Entry of a hantavirus into a host cell is negotiated by two membrane-anchored glycoproteins, Gn and Gc, which form a lattice decorating the lipid bilayer envelope of the mature virion. The Gc adopts a three-domain (domains I−III) class II fusion protein architecture and is postulated to associate closely with the Gn, linking adjacent Gn tetramers. Endosomal escape is mediated by the Gc in a process that involves engagement of the target membrane by the Gc-encoded fusion loop, followed by upward ‘zippering action’ conformational rearrangements of the transmembrane-anchored Gc domain III, which bring together host and viral membranes. Here we structurally characterize the epitope of mAb P-4G2, a potently neutralizing antibody derived following experimental infection of bank voles with Puumala virus (PUUV), a hantavirus responsible for one of the most frequently occurring hantaviral diseases, a mild form of HFRS known as nephropathia epidemica (NE).

To ascertain the position of the P-4G2 epitope in the context of the hantaviral envelope, we generated PUUV virus-like particles (VLPs) by transient expression of the PUUV genomic M-segment in mammalian cells. Cryo-ET of purified PUUV VLPs, in tandem with sub-tomogram averaging, revealed that the VLP surface displays the expected Gn−Gc spike architecture that can form locally ordered lattices, as observed in native hantavirions. Consistent with previous studies of hantavirus ultrastructure and Gc oligomerization, breakpoints exist in the (Gn−Gc)4 lattices. Previous studies have suggested that contacts between (Gn−Gc)4 spikes are mediated by Gc homo-dimers, while lattice breaks are expected to display Gc (‘lattice-free Gc’) molecules that are not integrated within the lattice assembly through Gc homo-dimer interactions. Drawing upon the fitting generated above, we used a 13.9 Å cryo-ET reconstruction of the lattice-incorporated (non-Fab P-4G2 treated) PUUV VLP surface to create a model of the higher-order (Gn−Gc)4 spike lattice. While the overall assembly of (Gn−Gc)4 spikes remain similar to that obtained from fitting into the cryo-ET reconstruction of an individual, Fab-treated glycoprotein spike fitting into the latticed reconstruction provides a structural basis for the formation of PUUV Gc homo-dimers at contact points between neighboring spikes, which closely resemble a crystallographically observed homo-dimer interface reported previously for HTNV Gc (Bignon et al., 2019; Guardado-Calvo et al., 2016). Furthermore, modeling of Fab P-4G2 binding onto the Gc homodimer demonstrates that neighboring epitopes are not mutually accessible for Fab binding in their lattice-integrated form, providing clues to how Fab P-4G2 recognition may be accompanied by dissociation of the Gc homodimer assembly.

>GPGETQNLNSGWTDTAHGSGIIPMRTDLELDFSLPSSASYTYRRQLQNPANEQEKIPFHLQISKQVIHAEIQHLGHWMDGTFNLKTAFHCYGSCEKYAYPWQTAGCFIEKDYEYESGWGCNPPDCPGVGTGCTACGVYLDKLKSVGKAFKIVSLRYTRKACIQLGTEQTCKSVDSNDCLVTTSVKVCLIGTVSKFQPSDTLLFLGPLEQGGLIFKQWCTTTCQFGDPGDIMSTPVGMKCPELNGSFRKKCAFATTPVCQFDGNTLSGYKRMIATKDSFQSFNVTEPHISASSLEWIDPDSSLRDHINVIVGRDLSFQDLSETPCQVDLATTSIDGAWGSGVGFNLVCSVSLTECSTFLTSIKACDSAMCYGSTTANLLRGQNTVHIVGKGGHSGSKFMCCHDTKCSSTGLVAAAPHLDRVTGYNQADSDKIFDDGAPECGISCWFTKSGEGTETSQVAPA[2x];>[2x]ETGELKIECPHTIGLGQGLVIGSVELPPVPLTQVESLKLESSCNFDLHTSTSSQQPFTKWTWEMKSDLAENTQASSTSFQTKSSEINLRGLCLVPPLVIETAARTRKTIACFDLSCNQTACQPTVFLIGPIQTCITTKSCLLGLGDQRIQVNYEKTYCVSGQLVEGVCFNPVHTMALSQPSHTYDIVTVMVRCFLIAKKVSTGDSMKLEKSFETLVQKTSCTGNGFQGYYICLVGSSSEPLYIPTLDDYRSAEVLSRMAFAPHGEDHDVEKNAISAMRIIGKVTGKAPSTESSDTIQGVAFSGNPLYTSTGVLTAKDDPVYIWAPGIIMEGNHSVCDKKTLPLTWTGFIPLPGEIEKTGTKHHHHHH> SSLPVPYKLPVSLSVGSCVIIKGTPIHSFINDPQLQVDFYTDMDEDSDIAFHFRVHFGNHVVMNRREFGIWMLEETTDYVPFEDGKQFELCIYVHYNEYEIKVNGIRIYGFVHRIPPSFVKMVQVSRDISLTSVCVCN

Galectin-13 (Gal-13, a.k.a. placental protein 13 or PP13) was first isolated from human placenta, and its gene has been mapped to chromosome 19q13.1, which is in close proximity to the galectin-4, -7, -10 and 1412 genes. As with all other galectins, Gal-13 adopts the typical “jelly-roll” fold formed by sandwiching two anti-parallel β-sheets that consist of six (S1-S6) and five (F1-F5) β-strands and a short α-helix connecting strands S2 and F5. Gal-13 crystallizes as a dimer with its subunit interface formed by the last five C-terminal residues (Val135, Cys136, Val137, Cys138, and Asn139) that are located within the F1 β-strand. We found that Gal-13 forms a homodimer structure that is stabilized primarily by the presence of two disulfide bonds, unlike the structures of other prototype galectins.

To test this hypothesis, we mutated Arg53 in Gal-13 to a histidine to assess whether we could restore lactose binding. Using the same conditions, however, we were unable to crystallize the R53H variant and had to use a different solution containing PEG 3350. However, we did not find lactose bound in the Gal-13 R53H mutant, even when the crystallization buffer contains 50 mM lactose. Nevertheless, the R53H variant does trap a molecule of glycerol at that site, and that trapped glycerol molecule is not observed when we flash cool a crystal of the R53H mutant in the absence of the glycerol cryoprotectant. Moreover, the C2, C3, O2, and O3 atoms of these two glycerol conformations occupy the same positions, whereas the C1 and O1 atoms are oriented differently. In one instance, the C1-O1 bond is oriented towards the conserved tryptophan (Trp72), and in the other, this bond is oriented towards Arg55. In this regard, the conformations of the two glycerol molecules in the R53H variant are different from those in Gal-3 and Gal-8.> MKKHLVVIAFCVLFASASAFAAKGTDSLKSSIEKYLKDKKAKVGVAVLGIEDNFKLNVNEKHHYPMQGTYKFHLALAVLDKLDKENISIDKKLFVKKSELLPNTWSPLRDKYPDGNVDLSISEILKATVSRSDNNGCDILFRFVGGTNKVHNFISKLGVKNISIKATEEEMHKAWNVQYTNWTTPDATVQLLKKFYKNEILSKNSYDYLLNTMIETTTGPKRLKGLLPDGTVVAHKTGSSDTNDKGITAATN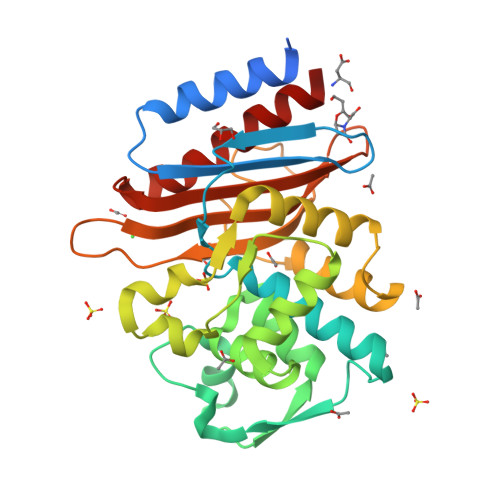DIGIITLPNGKHFAIAVYVSDSSEKSDVNEKIIAEICKSVWDYLVKD> ILKRCKTYDDCK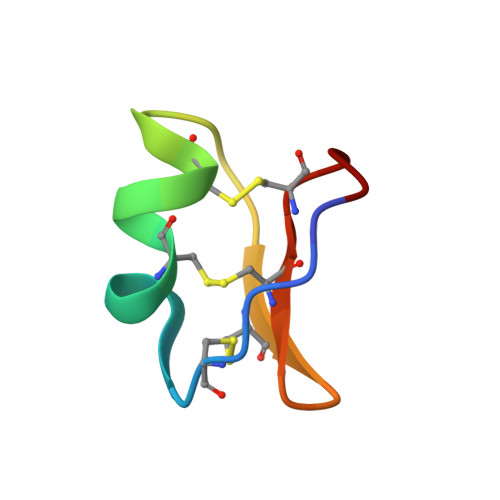DVCKARKGKCEFGICKCMIK> MASKKENLKSLFSNTRTRVIIIFTAALLIIAVVIGFFKIRGATTGSIAAAEVSTVPGGIQSIPGVLDPTAQYAKLQEEQNITQAQVAEKTGGSAIPTIIRTQALGEGVGVIGSQSGVGFAALAQEELGGPQRSLWIQELQDGSCSKSVITKVVNQGAQLTDLKAACSCVQLKDSGYGLQELEQVCECKELKSAGYNARQLKEAGYSAGRLRNCGFDACELRNAGFTAQEMKDGGFSDGELKGAGFSDAEIAKASGLPDGITADDVRKAGCGAAALAKLRQAGVSASAIRKISGCTAEQLKAAGYTAKELKDAGFSAADLRRAGFSAAELKDAGFTARDLLNAGFTPADLAKAGFSDAQIKAAQAELPPGITPQDVKNAGCDVEALKKEREAGVSAALIRQYAGCSAQALKAAGFTDADLANAGFTPAQISAATPLSDAEIKAAGCDPDKLKKLFSAGVSAKRIKELNGCSAEALKAAGYDAQSLLAAGFTPQELLAAGFTPKQLEDAGLNPVSIIADGRVADCSVESLKKARAAGVSALTIKQTLGCSAAALKAAGYTAKELKDAGFTAAELKAAGFSAKELKDAGFTAKELRDAGFSAQELKDVGFSAKDLKDAGFSAAELKAAGFTAAQLKAAGFSAKDLKDAGFSAAELKAAGFSAKELKDAGFSASDLKNAGFSAKELKDAGFSASDLKSAGFSASELKNAGYSADELKKAGYTSAELRNAGFSPQESAVAGLQGPDLQQLDSSITGIPSIPGATPRPTTSDAASSAEQLQAILQKQNEQLAEQKYQQEIQQRTSDMLTA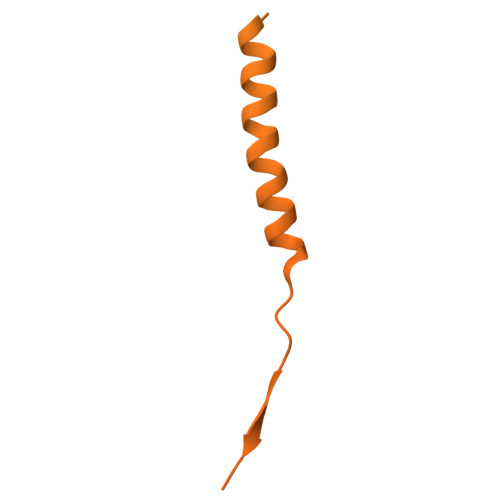ATQLVQDWKQVETQVYTEGTEETKTSGGESAVPGTGTGTGSNNQPVDQGAVSAQNQAIIKTGDIMFAVLDTSVNSDEPGPILATIVTGKLKGSKLIGSFNLPSNADKMVITFNTMSIPGAEKTISISAYAIDPNTARTALASRTNHHYLMRYGSLFASSFLQGFGNAFQSANTTITIGGTGGGNNITVANGVGRSTLENAVIGLATVGKAWSQQAQQLFNTPTTVEVYSGTGLGILFTQDVTTI>VEYRNWSKPQCQITGFAPFSKDNSIRLSAGGDIWVTREPYVSCDPVKCYQFALGQGTTLDNK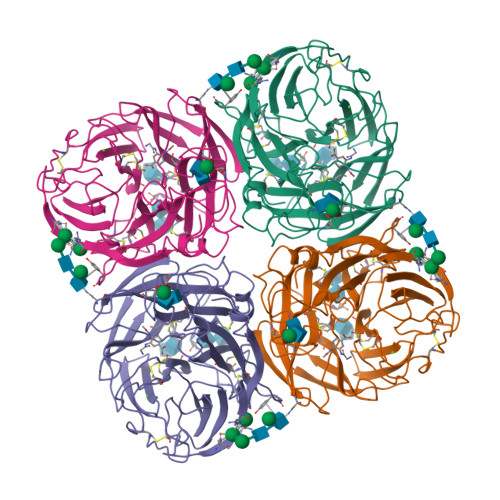HSNDTVHDRIPHRTLLMNELGVPFHLGTRQVCIAWSSSSCHDGKAWLHVCITGDDKNATASFIYDGRLVDSIGSWSQNILRTQESECVCINGTCTVVMTDGSASGRADTRILFIEEGKIVHISPLAGSAQHVEECSCYPRYPGVRCICRDNWKGSNRPVVDINMEDYSIDSSYVCSGLVGDTPRNDDRSSNSNCRDPNNERGTQGVKGWAFDNGNDLWMGRTISKDLRSGYETFKVIGGWSTPNSKSQINRQVIVDSDNRSGYSGIFSVEGKSCINRCFYVELIRGRKQETRVWWTSNSIVVFCGTSGTYGTGSWPDGANINFMPI[2x]>[2x]APKCIECHINIEMDPVLHDVFKLQVCKQCSK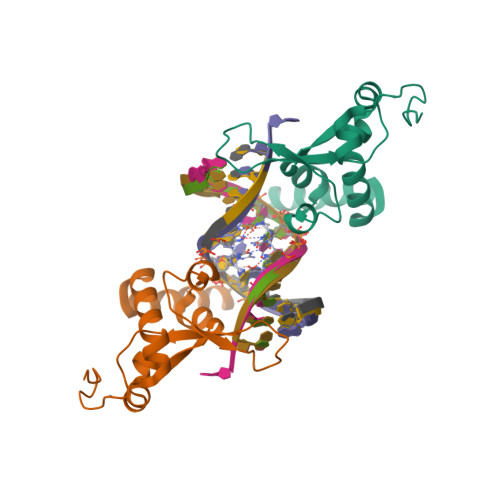EHPEKYALLTKTECKEDYFLTDPELNDEDLFHRLEKPNPHSGTFARMQLFVRCEVEAFAFKKWGGEEGLDEEWQRREEGKAHRR> ASPIGEGTFDDGPEGWVAYGTDGPLDTSTGALCVAVPAGSAQYGVGVVLNGVAIEEGTTYTLRYTATASTDVTVRALVGQNGAPYGTVLDTSPALTSEPRQVTETFTASATYPATPAADDPEGQIAFQLGGFSAD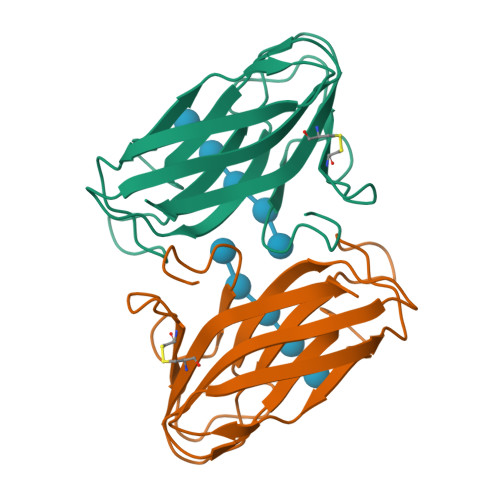AWTLCLDDVALDSE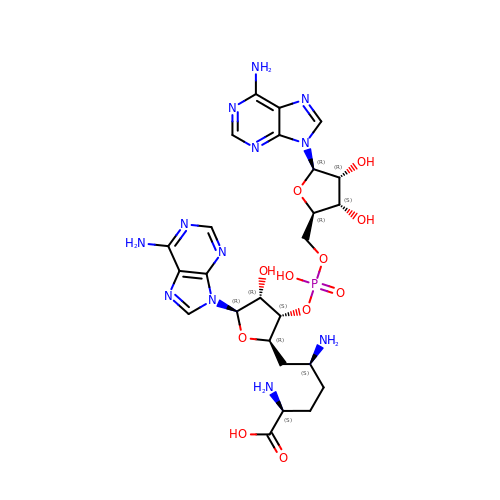(2~{S},5~{S})-6-[(2~{R},3~{S},4~{R},5~{R})-5-(6-aminopurin-9-yl)-3-[[(2~{R},3~{S},4~{R},5~{R})-5-(6-aminopurin-9-yl)-3,4-bis(oxidanyl)oxolan-2-yl]methoxy-oxidanyl-phosphoryl]oxy-4-oxidanyl-oxolan-2-yl]-2,5-bis(azanyl)hexanoic acid | C25 H35 N12 O11 P | XNBPELUUEBZQEC-PYTRVWNWSA-N>[2x]GPLGSYSHTATPAITLPSSGSANFAGVEYPLLPLDQHTPLLFQWFERNPSRFGENQIPIINTQQNPYLNNIINAAIIEKERTIGVLVDGNFSAGQKKALAKLEKQYENIKVIYNSDLDYSMYDKKLSDIYLENIAKIEAQPANVRDEYLLGEIKKSLNEVLKNNPEESLVSSHDKRLGHVRFDFYRNLFLLKGSNAFLEAGKHGCHHLQPGGGCIYLDADMLLTGKLGTLYLPDGIAVHVSRKGNSMS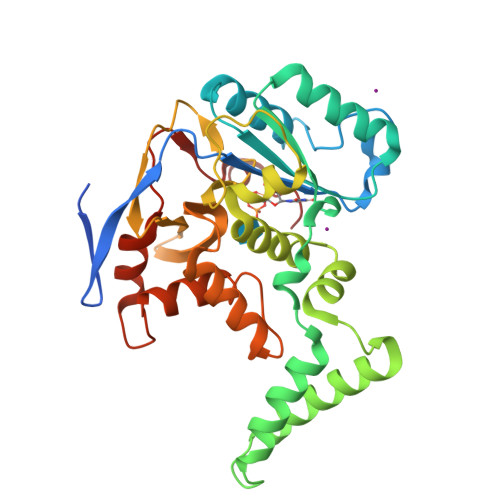LENGIIAVNRSEHPALKKGLEIMHSKPYGDPYIDGVCGGLRHYFNCSIRHNYEEFCNFIEFKHEHIFMDTSSLTISSWR>MKSSHHHHHHENLYFQSNASEFFWDVQKIQEISNVEEHSVVKCVTVNTSRLISQLNEELQDEESGVNFIVTQLQLLINNVYEKIQKSPGVPAHRSLMINLNFTRLKFSIAYWDILLERSLDLINGPSKTGARYFITEVTPVDRSRYVENNQYFLAFKANQRLTRNSVDMDEFIDFEILIKQIIFDLFKKNGIPDQDFEAILSRFHNLESLVVAFNE[4x];>ENKCIAVNENKVIENQKVIQSLCKNSHLDLIEQSYFGECDFIINHSTCVYKIQASRFMQL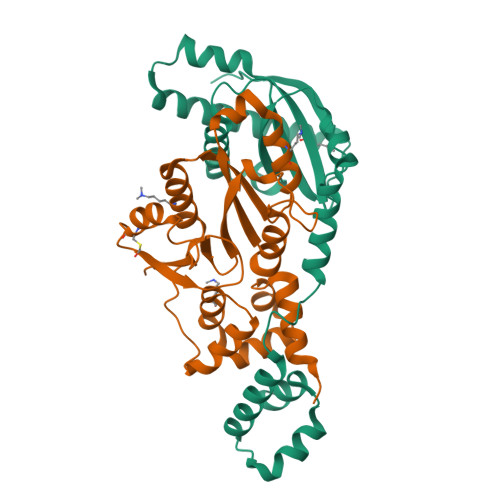RNNGSLHYDKAVNDLLTEFQRVIIIVEFSEIIQDVDPDLFWKIKLYLLNSRVDVFFIHETTDFFIDWMKYFIARWAFSYNDEKEKNIANADILLDLGFNILLVRKIFQTYSLEEFFMAIIKEESKAVKMLTVSQMTRLKKLLTLEW[4x]>QGHMRATNVTYQAHHVSRNKRGQVVGTRGGFRGCTIWLTGLSGAGKTTVSMALEEYLVCHGIPCYTLDGDNIRQGLNKNLGFSPEDREENVRRIAEVAKLFADAGLVCITSFISPYTQDRNNARQIHEGASLPFFEVFVD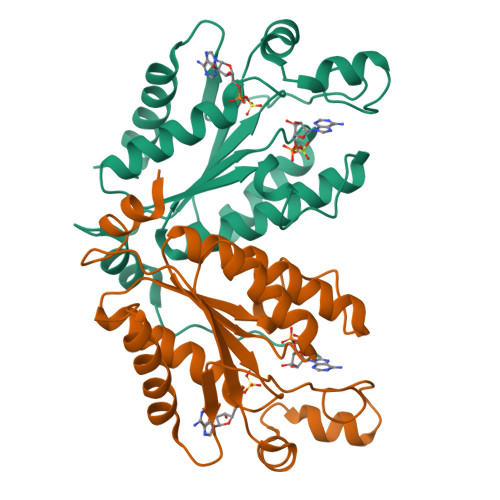APLHVCEQRDVKGLYKKARAGEIKGFTGIDSEYEKPEAPELVLKTDSCDVNDCVQQVVELLNERDILP[8x]>[5x]MAELPPGRLATTEDYFAQQAKQAVTPDVMAQLAYMNYIDFISPFYSRGCSFEAWELKHTPQRVIKYSIAFYAYGLASVALIDPKLRALAGHDLDIAVSKMKCKRVWG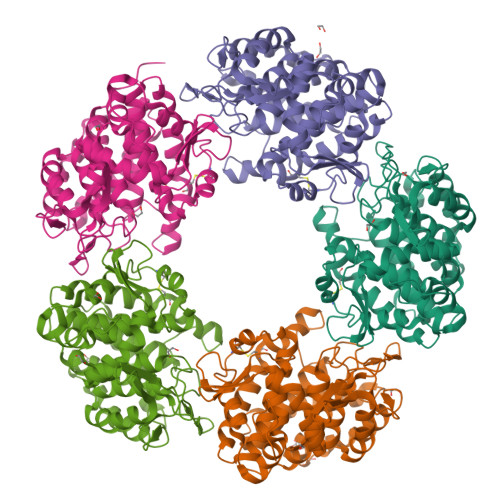DWEEDGFGTDPIEKENIAYKGHLNLMYGLYQLVTGSRRYEAEHAHLTRIIHDEIAANPFAGIVCEPDNYFVQCNSVAYLSLWVYDRLHGTDYRAATRAWLDFIQKDLIDPERGAFYLSYHPESGAVKPWISAYTTAWTLAMVHGMDPAFSERYYPRFKQTFVEVYDEGRKARVRETAGTDDADGGVGLASAFTLLLAREMGDQQLFDQLLNHLEPPAKPSIVSASLRYEHPGSLLFDELLFLAKVHAGFGALLRMPPPAAKLAGK3-[[4-oxidanyl-1-[(3~{S},4~{S})-3-phenyl-1-(phenylmethyl)piperidin-4-yl]carbonyl-piperidin-4-yl]methyl]quinazolin-4-one 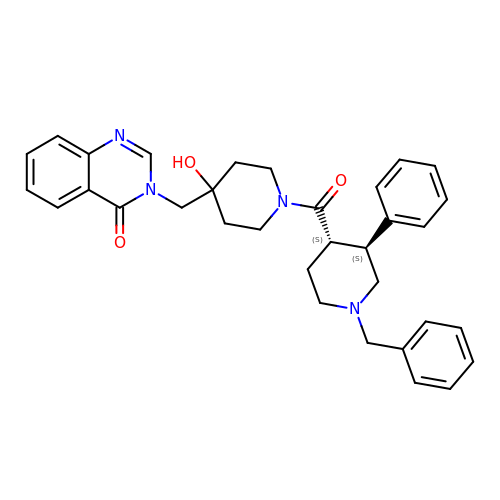| C33 H36 N4 O3 | IVQSXYDLXVYPHO-LMSSTIIKSA-N>[8x]FNLPLGNYKK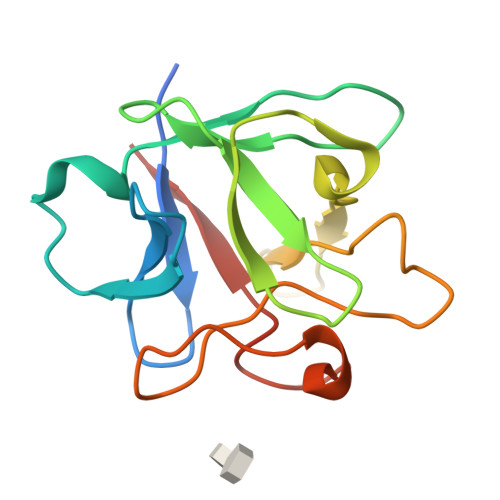PKLLYCSNGGYFLRILPDGTVDGTKDRSDQHIQLQLAAESIGEVYIKSTETGQFLAMDTDGLLYGSQTPNEECLFLERLEENHYNTYISKKHAEKHWFVGLKKNGRSKLGPRTHFGQKAILFLPLPVSSD>[2x]MGGSHHHHHHGMAS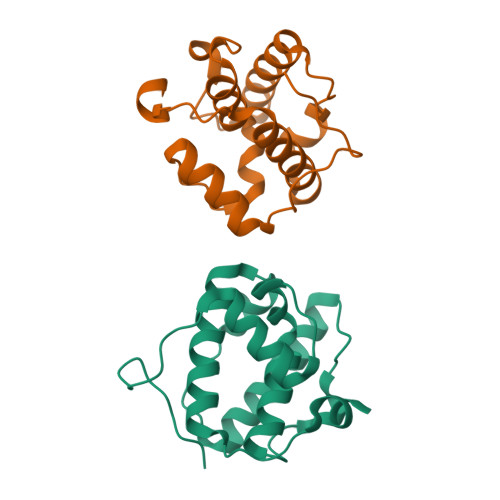AVNVYSTSVTSDNLSRHDMLAWINESLQLNLTKIEQLCSGAAYCQFMDMLFPGSIALKKVKFQAKLEHEYIQNFKILQAGFKRMGVDKIIPVDKLVKGKFQDNFEFVQWFKKFFDANYDGKDYDPVAARQGQETAVAPS pyren-1-yl 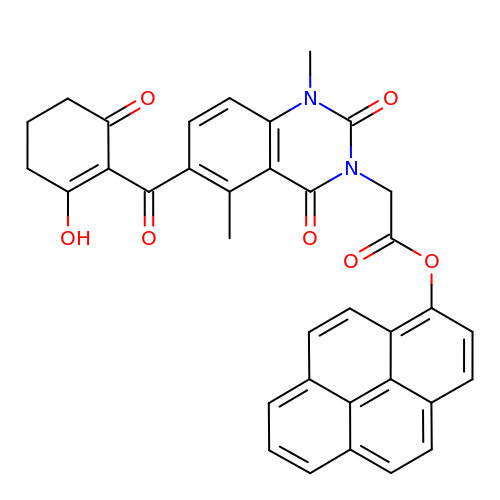2-[1,5-dimethyl-2,4-bis(oxidanylidene)-6-(2-oxidanyl-6-oxidanylidene-cyclohexen-1-yl)carbonyl-quinazolin-3-yl]ethanoate | C35 H26 N2 O7 | SFJMSYJSOPJDJE-UHFFFAOYSA-N>MIVLFVDFDYFYAQVEEVLNPSLKGKPVVVCVFSGRFEDSGAVATANYEARKFGVKAGIPIVEAKKILPNAVYLPMRKEVYQ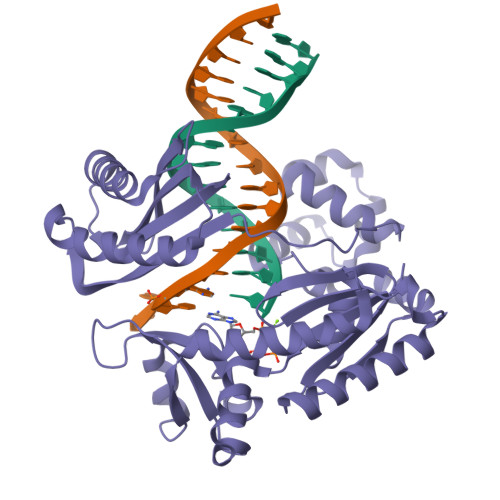QVSSRIMNLLREYSEKIEIASIDEAYLDISDKVRDYREAYNLGLEIKNKILEKEKITVTVGISKNKVFAKIAADMAKPNGIKVIDDEEVKRLIRELDIADVPGIGNITAEKLKKLGINKLVDTLSIEFDKLKGMIGEAKAKYLISLARDEYNEPIRTRVRKSIGRIVTMKRNSRNLEEIKPYLFRAIEESYYKLDKRIPKAIHVVAVTEDLDIVSRGRTFPHGISKETAYSESVKLLQKILEEDERKIRRIGVRFSKFI[4x]>GPGSMSEKGRLFTSESVTEGHPDKICDAVSDSVLDALLAADPRSRVAVETLVTTGQVHVVGEVTTTAKEAFADITNIVRERILDIGYDSSDKGFDGASCGVNIGIGAQSPDIAQGVDTAHEARVEGAADPLDAQGAGDQGLMFGYAINDTPELMPLPIALAHRLSRRLTEVRKNGVLPYLRPDGKTQVTIAYEDRVPVRLDTVVISTQHADDIDLVKTLDPDIREQVLKTVLDDLAHDTLDASAVRVLVNPTGKFVLGGPMGDAGLTGRKIIVDTYGGWAR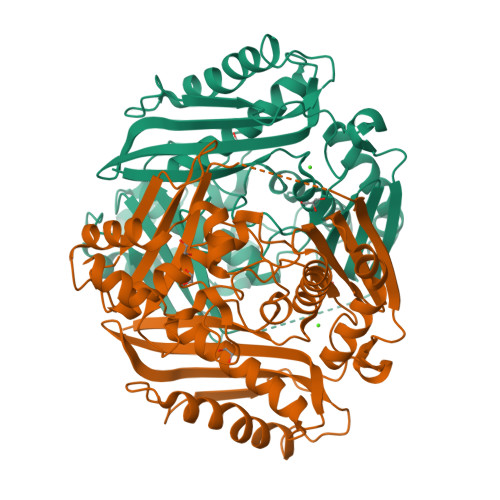HGGGAFSGKDPSKVDRSAAYAMRWVAKNVVAAGLAERVEVQVAYAIGKAAPVGLFVETFGSEAVDPVKIEKAIGEVFDLRPGAIIRDLNLLRPIYAPTAAYGHFGRTDVDLPWERLDKVDDLKRAI[2x]>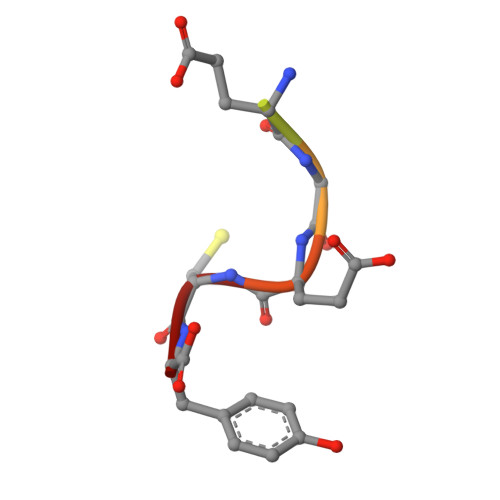 GEEEGECY> EWTGDARDGMFSGVVITQFHTGQIDNKPYFCIEGKQSAGSSISACSMKNSSVWGASFST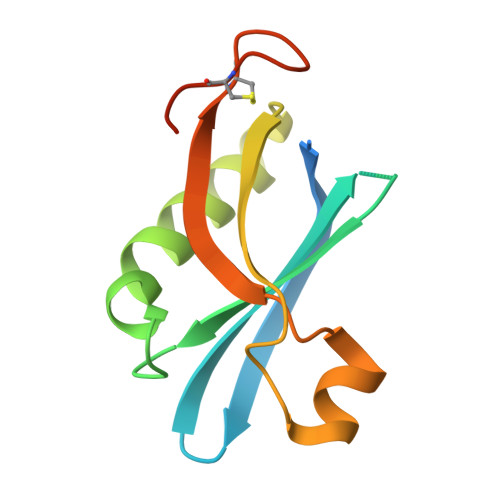LYNQALYFYTTGQPVRIYYEPGVWTYPPFVKALTSNALVGLSTCTTSTECFGPDRKKNSLE>[2x]GPGSEFKV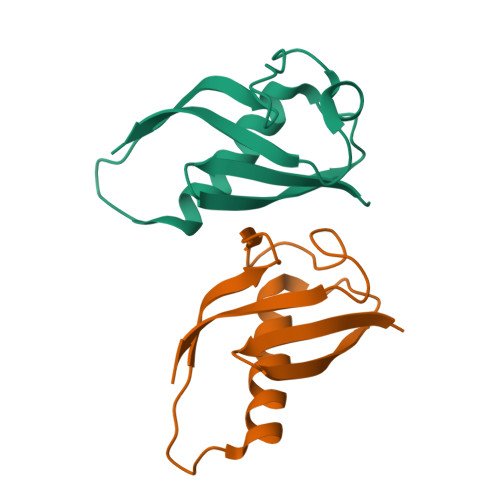TVCFGRTRVVVPCGDGRMKVFSLIQQAVTRYRKAVAKDPNYWIQVHRLEHGDGGILDLDDILCDVADDKDRLVAVFDEQD>[2x]GSKVVKFSYMWTINNFSFCREEMGEVIKSSTFSSGANDKLKWCLRVNPKGLDEESKDYLSLYLLLVSCPKSEVRAKFKFSILNAKGEETKAMESQRAYRFVQGKDWGFKKFIRRGFLLDEANGLLPDDKLTLFCEVSVVQDSVNISGQNTMNMVKVPECRLA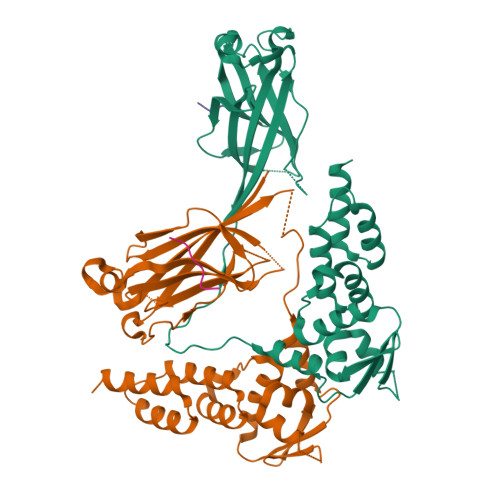DELGGLWENSRFTDCCLCVAGQEFQAHKAILAARSPVFSAMFEHEMEESKKNRVEINDVEPEVFKEMMCFIYTGKAPNLDKMADDLLAAADKYALERLKVMCEDALCSNLSVENAAEILILADLHSADQLKTQAVDFINYHATDVLETSG;>[2x]DEVTSTT>MASTDYHVDLTNCDREPIHIPGYIQPHGCLIACDNAMRMVLRHSENCGELLGLEGDLNGRTAEDVLGKRLVHDLRNALTVTGKTTRPAMLPAMETSDGRSFDISLHRYKSTTIIEFEPSDSDTQPLGTARKMVDRIREADSVESLISRTTRLVKATLGYDRVLIYRFEEDGAGKVVSEAKQPELESFLGQYFPASDIPQQARALYLKNTLRIISDASGTPIPVLPAVDVSGEPLDLSYAHLRNFSPIHCEYLRNMGVAASMSISVIVDDALWGLIVCHHCSPRVLSMPVRIAAAMFGEFFSMFLQVLKQKRRLDTINHAHAALDRFLRLAAHRANLEELLVDSFQDFARLIPCDGVGLWVGNNWHGHGATPPHDAIPRLARFVASVSEGRVWATHALSQAIPEAEIYADTAAGMLAIPISQVKSDYLLFFRKEIVQNLNWAGNPEKSYETGPMGDRLTPRKSFAIWKES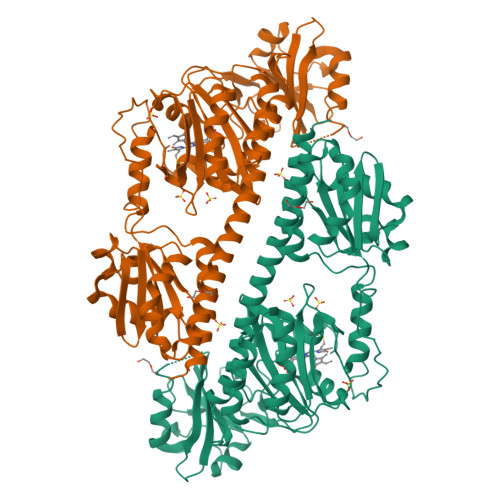VRLQAQPWSEADREIAETARIALVGVAFHHSELMAGLEYKHHHHHH[2x]> GPLGSDPAQIVLTIPETEYIYGPLNRSFRKHLPNVPVSRSLPVTIDKLTFHYGDYEQLDMDQLMSNQLYHANSYIYRKAIIRKHYLSHTIHSYVVKNRESILNRAFLESFNIDVDYAEFLD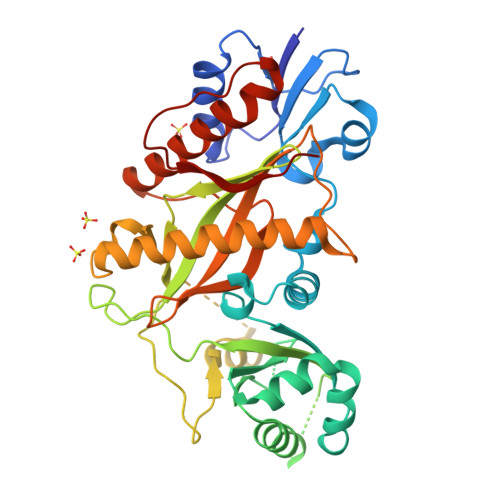DALDENWELRQELESKEKWWILKPSMSDKGQGIRIFKTIEQLQAIFDSFEEDETDDEDTETNTNKVATSQLRHFIVQEYLHNPLLLSEAHGRKFHIRCYVTCSGDLQVFVYDRMLALFAPNKFVPPTEEYDVLDIEQLACHLTNTCLQTDDDIKSNSVIEFDALKDIPSHRREEIRTQIHEAVSELFKAAVNVDRLNFRPLKNSLETFGFDFLVDSDYQVKLLEVNAFPDFKQTGDDLKNLIDELFDDVVSICVRPMFNLPPLHHQHSKFVEVLKLKSNDW>[2x]VAPKPIVDIDGKPVLY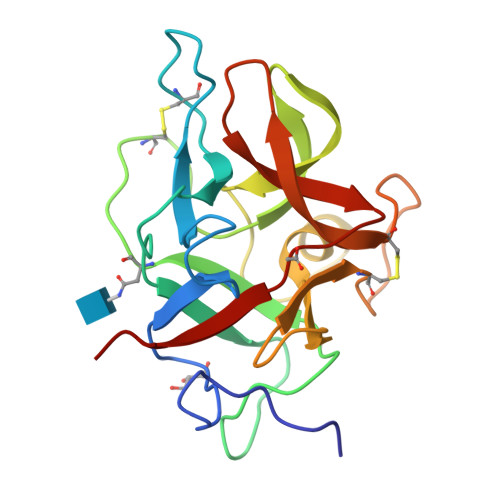GVDYFVVSAIWGAGGGGLTVYGPGNKKKCPLSVVQDPFDNGEPIIFSAIKNVKDNIVRESVDLNVKFNITINCNETTAWKVDRFPGVIGWTVTLGGEKGYHGFESTHSMFKIKKAGLPFSYKFHFCPSYPRTRLIPCNNVDIFFDKYRIRRLILTNDAKEFVFIKTNR> GSMAAQRRSLLQSEQQPSWTDDLPLCHLSGVGSASNRSY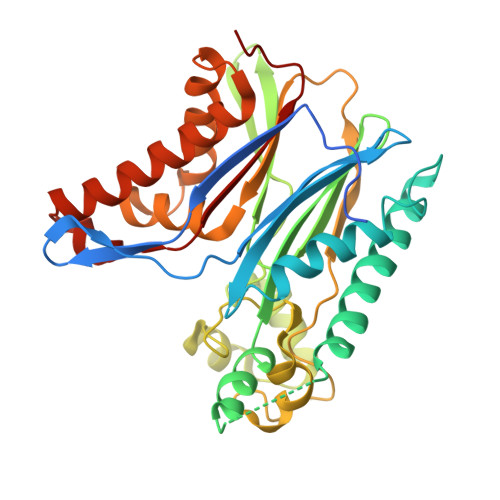SADGKGTESHPPEDSWLKFRSENNCFLYGVFNGYDGNRVTNFVAQRLSAELLLGQLNAEHAEADVRRVLLQAFDVVERSFLESIDDALAEKASLQLERLKTLEREISGGAMAVVAVLLNNKLYVANVGTNRALLCKSTVDGLQVTQLNVDHTTENEDELFRLSQLGLDAGKIKQVGIICGQESTRRIGDYKVKYGYTDIDLLSAAKSKPIIAEPEIHGAQPLDGVTGFLVLMSEGLYKALEAAHGPGQANQEIAAMIDTEFAKQTSLDAVAQAVVDRVKRIHSDTFASGGERARFCPRHEDMTLLVRNFGYPLG> MDEEREKLKEKLKEVLRRAKEAKKKGDKEKLIELAYEAAALAAWIIHKDSNDDEIVELAKEALKLVLEAAKEAKKNGDKEKLIKLAYLAAAVAAWIIHTDGDDDEIVELAKEALKLVLEAAKEAKKNGDKE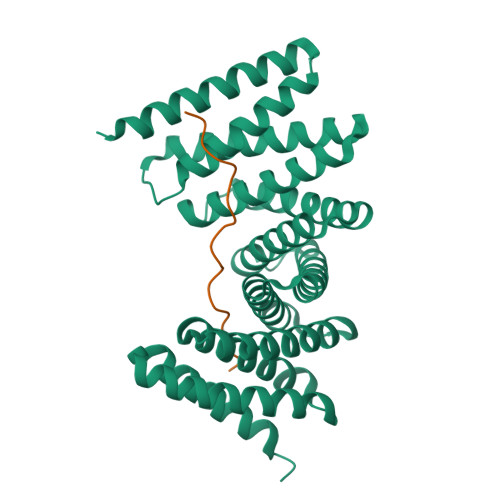KLIKLAYLAAAVAAWIITTDGDDDEIVELAKEALKLVLEAAKEAKKNGDKEKLIKLAYLAAAVAAWIIHTDGDDDEIVELAKEALKLVLEAAKEAKKNGDKEKLIKLAYLAAAVAAWIITTDGDDEEIVELAKEALKLVKEAAEEAEKQGDEELREKLRYLSEAVREWIERND;> PLPPLPPLPPLPPLPPLPP>[8x]ARV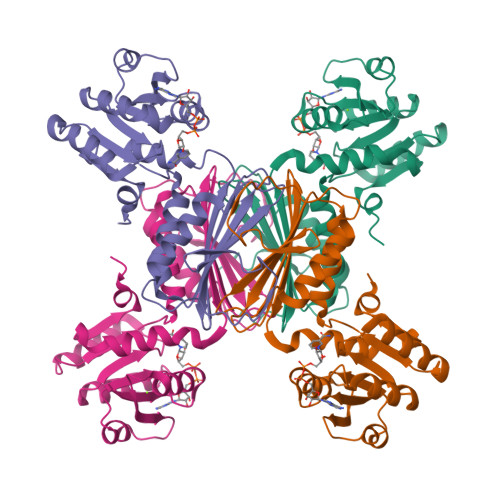GVLGAKGKVGATMVRAVAAADDLTLSAELDAGDPLSLLTDGNTEVVIDFTHPDVVMGNLEFLIDNGIHAVVGTTGFTAERFQQVESWLVAKPNTSVLIAPNFAIGAVLSMHFAKQAARFFDSAEVIELHHPHKADAPSGTAARTAKLIAEARKGLPPNPDATSTSLPGARGADVDGIPVHAVRLAGLVAHQEVLFGTEGETLTIRHDSLDRTSFVPGVLLAVRRIAERPGLTVGLEPLLDLH>[3x]MPEGPELHLASQFVNEACRALVFGGCVEKSSVSRNPEVPFESSAY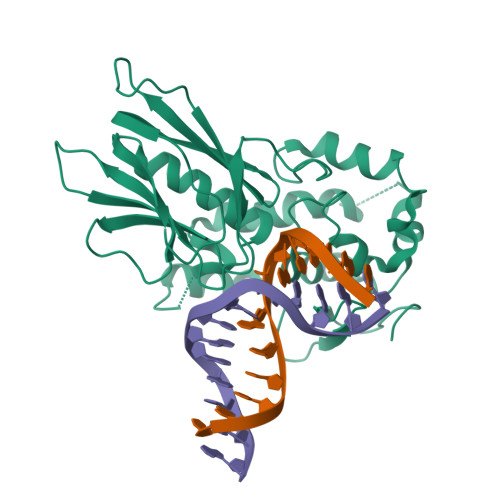RISASARGKELRLILSPLPGAQPQQEPLALVFRFGMSGSFQLVPREELPRHAHLRFYTAPPGPRLALCFVDIRRFGRWDLGGKWQPGRGPCVLQEYQQFRENVLRNLADKAFDRPICEALLDQRFFNGIGNYLRAEILYRLKIPPFEKARSVLEALQQHRPSPELTLSQKIRTKLQNPDLLELCHSVPKEVVQLGGKGYGSESGEEDFAAFRAWLRCYGMPGMSSLQDRHGRTIWFQGDPGPLAPKGRKSRKKKSKATQLSPEDRVEDALPPSKAPSRTRRAKRDLPKRTATQRPEGTSLQQDPEAPTVPKKGRRKGRQAASGHCRPRKVKADIPSLEPEGTSASAALGHHHHHH The cyclic oligonucleotide-based antiphage signalling system (CBASS) and the pyrimidine cyclase system for antiphage resistance (Pycsar) are antiphage defence systems in diverse bacteria that use cyclic nucleotide signals to induce cell death and prevent viral propagation. Here we show that phages encode anti-CBASS (Acb) and anti-Pycsar (Apyc) proteins that counteract defence by specifically degrading cyclic nucleotide signals that activate host immunity. Using a biochemical screen of 57 phages in Escherichia coli and Bacillus subtilis, we discover Acb1 from phage T4 and Apyc1 from phage SBSphiJ as founding members of distinct families of immune evasion proteins. We confirmed the critical role for Apyc1 metal-coordinating residues and identified E74 and Y112 from the opposing protomer as further catalytic residues required for cCMP hydrolysis and release of the reaction product 5′-CMP. Together, these findings demonstrate that Acb1 and Apyc1 constitute separate families of immune evasion proteins and explain the distinct reaction mechanisms that degrade CBASS or Pycsar cyclic nucleotide signals.

To compare mechanisms of anti-CBASS and anti-Pycsar evasion, we determined the crystal structure of Apyc1 from the phage Bsp38 (2.7 Å) as well as structures of Paenibacillus Apyc1 proteins (1.5 Å and 1.8 Å). Structures of Apyc1 reveal a metal-dependent cyclic NMP phosphodiesterase that uses relaxed specificity to target Pycsar cyclic pyrimidine mononucleotide signals. We identified 107 proteins related to Apyc1 present in phage genomes and also found many closely related bacterial proteins encoded in diverse bacterial orders. Similar to SBSphiJ Apyc1, closely related phage and bacterial Apyc1-like proteins cleaved cyclic mononucleotides with broad specificity. The observation of Apyc1 homologues encoded in bacteria may be explained by the presence of cryptic prophages present in bacterial genomes, but also raises the intriguing possibility that host Apyc1 enzymes may play a role in regulating Pycsar defence or other cNMP-based signalling systems. Structural comparison of Apyc1 and B. subtilis YhfI also reveals that Apyc1 enzymes contain an extended loop that reaches into the nucleotide-binding pocket, potentially enabling stable binding of smaller cyclic pyrimidine substrates.

>[2x]SSLQIQMIGTGSAFAKKFYNNNALVKCNGFQLLIDCGVTAPRALHELGVPITGIDGILITHIHADHVGGIEEFAFRLKYKYGMTIKLFVPAALVNPLWDHSLRGGLENKAEGLEQLADYFDVVALEEAVVHEIHPGLTVELVRSQHIAGKASYSLLLNNLLFYSSDARFNYAQLVELSTSGRCKYILHDCQLAEPAAVHATLNELLTLPEAVQEMIMLMHYDDEMEQFIGKSGKMSFMQQHKTYSFTEAT> GPGSEFQECAVCGWALPHNRMQALTSCECTICPDCFRQHFTIALKEKHITDMVCPACGRPDLTDDTQLLSYFSTLDIQLRE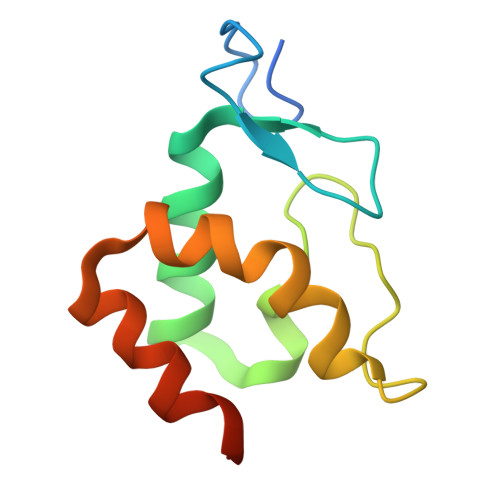SLEPDAYALFHKKLTEGVLMRD>MGSSHHHHHHGSSNILIINGAKKFAHSNGQLNDTLTEVADGTLRDLGHDVRIVRADSDYDVKAEVQNFLWADVVIWQMPGWWMGAPWTVKKYIDDVFTEGHGTLYASDGRTRKDPSKKYGSGGLVQGKKYMLSLTWNAPMEAFTEKDQFFHGVGVDGVYL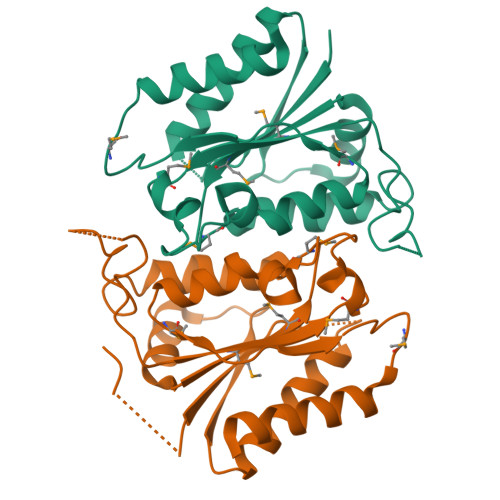PFHKANQFLGMEPLPTFIANDVIKMPDVPRYTEEYRKHLVEIFG[4x]> GSHMERPESELIRQSWRVVSRSPLEHGTVLFARLFALEPSLLPLFQYNGRQFSSPEDSLSSPEFLDHIRKVMLVIDAAVTNVEDLSSLEEYLTSLGRKHRAVGVRLSSWSTVGESLLYMLEKSLGPDFTPATRTAWSRLYGAVVQAMSRGWDGE

To investigate the correlation between mechanical properties and functional efficiency in proteins, we selected neuroglobin (Ngb), a hexacoordinated heme protein, which is expressed in the neurons of vertebrates and is involved in neuroprotection in hypoxic conditions and protects brain from stroke. Ngb folds like all globins with a bundle of eight helices termed A to H, and a heme hexacoordinated in both ferric and ferrous forms by the imidazole side chain of the distal and proximal histidines (His 64 and His 96 respectively). The structures of human and murine Ngb present a large internal cavity behind the heme, that is connected to the surface through a tunnel, forming a pathway toward the heme for gaseous ligands (O2, CO, NO). Like many recently discovered globins, Ngb is characterized by endogenous heme iron hexacoordination in the absence of external ligands.

The effects of high-pressure on the structure of the F106W mutant shed light on the role of Phe 106 and helix G. This mutant is endowed with an enhanced barrier to heme sliding, as indicated by decreased CO affinity. Between F106W HP-310 and F106W AP, the main segments affected by pressure are the BC and CD loops, the N-terminal segment of helices F and G, and especially the second half of helix H which is shifted by more than 1 Å toward helix G which carries the F106W mutation. The protein mean B-factors are considerably raised by pressure, which could explain why this mutant is more sensitive to pressure than WT Ngb. The residues whose B-factors present a relevant increase with pressure (more than 15 Å2) are mostly located at the back of the protein, while the residues whose B-factors are moderately increased by pressure (less than 5 Å2) are mainly located close to the heme. The effect of pressure seems to be the opposite of what was previously observed in WT Ngb under pressure. There is a shrinkage of its volume between the HP-310 and AP structures by 8%. In particular, the tunnel disappears already at 280 MPa and site I disappears at 310 MPa, while site II remains insensitive to pressure (data not shown). The force constant variation profiles between F106W HP-310 and F106W AP presents four peaks, three of them correspond to residues belonging to the WT mechanical nucleus, and one corresponds to Met 69, which lies away from the main cavity. The HP structures reveal that the flexibility of the extended FG loop is restrained by the presence of a tryptophan at position 106, with no particular flexibility of Val 99.>[2x]MAETSLPELGGEDKATPAPSILELEEL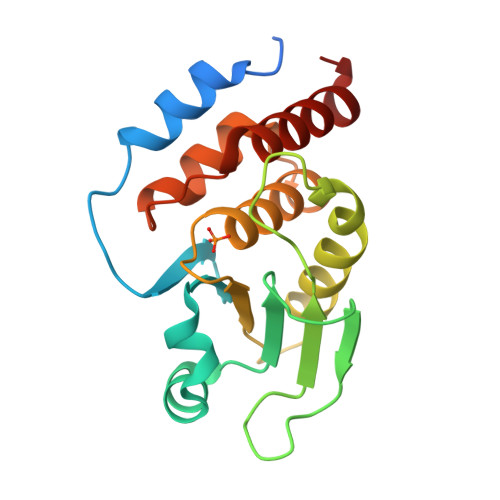LRAGKSSASRVDEVWPNLFIGDAATANNRFELWKLGITHVLNAAHKGLYAQGGPDFYGSSVSYLGVPAHDLPDFDISAYFSSAADFIHRALNTPGAKVLVHSVVGVSRSATLVLAYLMLHQRLSLRQAVITVRQHRWVFPNRGFLHQLARLDQQLRGA>[2x]GPAMNSVFSGLDMLILLPYERRGTRLVVEDYRPDHIYCIGADFGKNQDYSVFSVLDLDTGAIACLERMNGATWSDQVARLKALSEDYGHAYVVADTWGVGDAIAEELD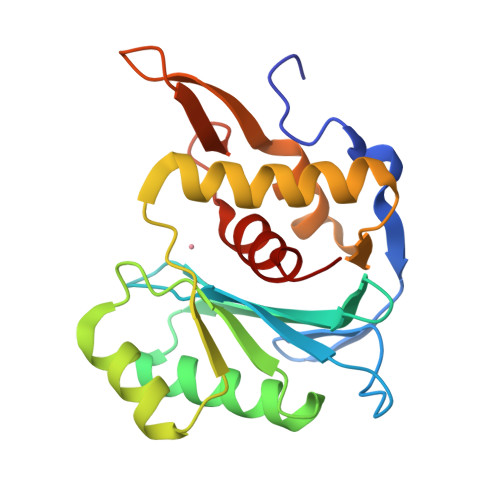AQGINYTPLPVKSSSVKEQLISNLALLMEKGQVAVPNDKTILDELRNFRYYRTASGNQVMRAYGRGHDDIVMSLALAYSQYEG>[3x]GSIIEMRDVVKKYDNGTTALRGVSVSVQPGEFAYIVGPSGAGKSTFIRSLYREVKIDKGSLSVAGFNLVKIKKKDVPLLRRSVGVVFQDYKLLPKKTVYENIAYAMEVIGENRRNIKRRVMEVLDLVGLKHKVRSFPNELSGGEQQRIAIARAIVNNPKVLIADEPTGNLDPDNSWEIMNLLERINLQGTTILMATHNSQIVNTLRHRVIAIENGRVVRDESKGEYGYDD

FtsEX is a membrane complex widely conserved across diverse bacterial genera and involved in critical processes such as recruitment of division proteins and in spatial and temporal regulation of muralytic activity during cell division or sporulation. The component FtsX is an integral membrane protein, whereas FtsE is an ATPase and is required for the transmission of a conformational signal from the cytosol through the membrane to regulate the activity of cell wall hydrolases in the periplasm. Here, we provide the first three-dimensional (3D) structure of FtsE from the notorious pathogen S. pneumoniae, and we show that it presents all the conserved structural motifs of the NBD members of the ABC transporter family. The nucleotide-binding site is located in lobe I near the interface between the two lobes and presents the nucleotide sandwiched between the Walker A and B motifs.

Two different crystal forms in complex with ADP were obtained in the same crystallization conditions belonging to two different space groups, P 1 and P 21. P 1 crystals contain one molecule per asymmetric unit and diffract up to 1.36 Å resolution, while P 21 crystals contain three molecules per asymmetric unit and diffract up to 1.57 Å resolution. In both P 1 and P 21, the resulting structures correspond to monomeric FtsE and provided excellent electron density for all 230 amino acid residues of the protein. Structural comparison of the four independent FtsE structures reported here (one monomer from the P 1 crystal form and three others, M1, M2, and M3, from the P 21 crystal form associated with chain IDs A, B, and C, respectively) reveals significant differences among them. The fourth region (R4, residues 101 to 115) affects the C-terminal part of α3, which is even partially unfolded in monomer 1, resulting in a longer coil loop that protrudes from the monomer structure. Morphing between the two most structurally different FtsE monomers (monomer from P 1 and monomer 1 from P 21) illustrates the kind of movements observed between lobes I and II of FtsE. The distance and the angle between the two lobes fluctuate up to ∼4 Å and 9° (considering N157 as the hinge between the two lobes), respectively, revealing an unexpected intramolecular breathing motion within the FtsE monomer. In addition, two extra ADP molecules were also found in the P 21 crystal form. They increase crystal contacts but are not located in sites with physiological relevance in other ATPases.> GSGEPREEAGALGPAWDESQLRSYSFPTRPIPRLSQSDPRAEELIENEEPVVLTDTNLVYPALKWDLEYLQENIGNGDFSVYSASTHKFLYYDEKKMANFQNFKPRSNREEMKFHEFVEKLQDIQQRGGEERLYLQQTLNDTVGRKIVM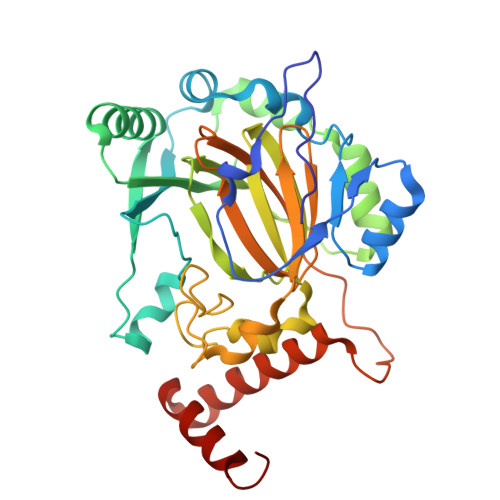DFLGFNWNWINKQQGKRGWGQLTSNLLLIGMEGNVTPAHYDEQQNFFAQIKGYKRCILFPPDQFECLYPYPVHHPCDRQSQVDFDNPDYERFPNFQNVVGYETVVGPGDVLYIPMYWWHHIESLLNGGITITVNFWYKGAPTPKRIEYPLKAHQKVAIMRNIEKMLGEALGNPQEVGPLLNTMIKGRYN P-FLUORO-7-BENZYL GUANINE MONOPHOSPHATE | C17 H20 F N5 O8 P | 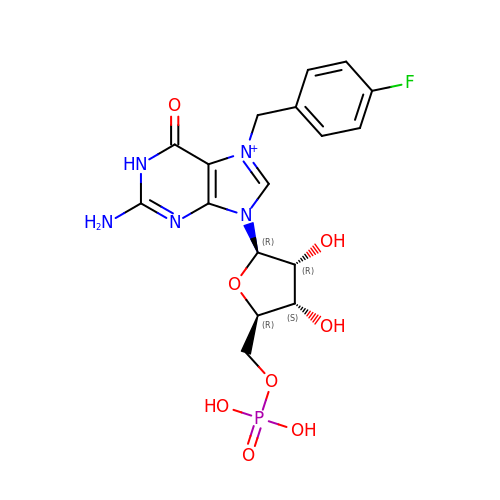VLABRVWLURSKLS-XNIJJKJLSA-O>[2x]GPGADGWLELESDPGLFTLLLKDFGCHDVQVEEVYDLQKPIESPYGFIFLFRWIEERRARRKIVETTAEIFVKDEEAISSIFFAQQVVPNSCATHALLSVLLNCNENNLQLGDTLSRLKTHTKGMSPENKGLAIGNTPELACAHNSHAMPQARRRLERTGAGVSSCRFTGEAFHFVSFVPINGQLFELD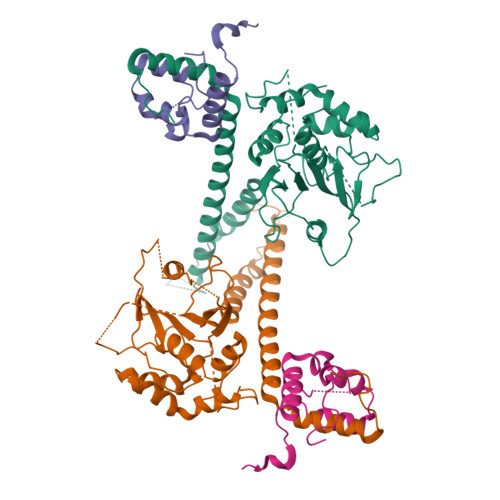GLKPYPMNHGGWEDSEDWTDKFRRVMAERLGIATGEQDIRFNLMAVVPDRRIAITHKLKMLRTNQAIVSGTLQKLLKADEQGESGNGDSQRPDTPTTLLEPSAFTARDLQSLLKNLDTEIAINEQHLADENDRRHMFKVDASRRTHNYDKFICTFLSMLAHQGVLGELVSQHLLPS;>[2x]DGKIDLETPDSILASTNLRALLNKQTFSLLPPLYQYNLIQLLPSVDREASELEQPSSSASGGSPSEAIRLSASCLNNEFFARACLEWRERLSEGEFTPENQLKLKTEAEREKNKLDPWKLKHFEPFWGEKNSRG> QECTKFKVSSCRECIESGPGCTWCQKLNFTGPGDPDSIRCDTRPQLLMRGCAADDIMDPTSLAETQEDHNGGQKQLSPQKVTLYLRPGQAAAFNVTFRRAKGYPIDLYYLMDLSYSMLDDLRNVKKLGGDLLRALNEITESGRIGFGSFVDKTVLPFVNTHPDKLRNPCPNKEKECQPPFAFRHVLKLTNNSNQFQTEVGKQLISGNLDAPEGGLDAMMQVAACPEEIGWRNVTRLLVFATDDGFHFAGDGKLGAILTPNDGRCHLEDNLYKRSNEFDYPSVGQLAHKLAENNIQPIFAVTSRMVKTYEKLTEIIPKSAVGELSEDSSNVVQLIKNAYNKLSSRVFLDHNALPDTLKVTYDSFCSNGVTHRNQPRGDCDGVQINVPITFQVKVTATECIQEQSFVIRALGFTDIVTVQVLPQCECRCRDQSRDRSLCHGKGFLECGICRCDTGYIGKNCECQTQGRSSQELEGSCRKDNNSIICSGLGDCVCGQCLCHTSDVPGKLIYGQYCECDTINCERYNGQVCGGPGRGLCFCGKCRCHPGFEGSACQCERTTEGCLNPRRVEC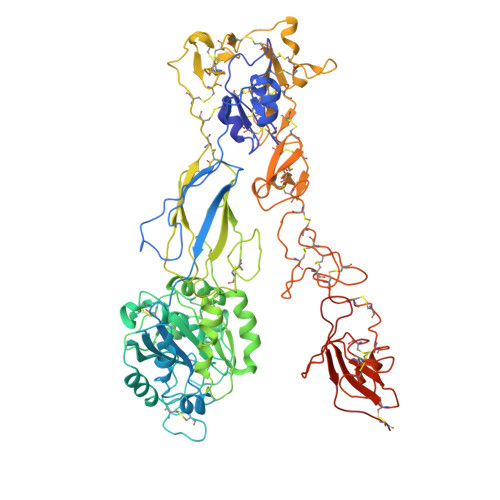SGRGRCRCNVCECHSGYQLPLCQECPGCPSPCGKYISCAECLKFEKGPFGKNCSAACPGLQLSNNPVKGRTCKERDSEGCWVAYTLEQQDGMDRYLIYVDESRECVAGPDGCGENLYFQ>[8x]MVQASGHRRSTRGSKMVSWSVIAKIQEILQRKMVREFLAEFMSTYVMMVFGLGSVAHMVLNKKYGSYLGVNLGFGFGVTMGVHVAGRISGAHMNAAVTFANCALGRVPWRKFPVYVLGQFLGSFLAAATIYSLFYTAILHFSGGQLMVTGPVATAGIFATYLPDHMTLWRGFLNEAWLTGMLQLCLFAITDQENNPALPGTEALVIGILVVIIGVSLGMNTGYAINPSRDLPPRIFTFIAGWGKQVFSNGENWWWVPVVAPLLGAYLGGIIYLVFIGSTIPREPLKLEDSVAYEDHGITVLPKMGSHEPTISPLTPVSVSPANRSSVHPAPPLHESMALEHF

pmcAquaporins (AQPs) are integral membrane proteins facilitating the flux of water (orthodox AQPs) and/or small neutral solutes such as glycerol, arsenite, and urea (aquaglyceroporins) across the lipid bilayer of cells. The human genome encodes four aquaglyceroporins AQP3, AQP7, AQP9, and AQP10 and recently AQP7 was identified as a novel regulator of breast cancer. The model shows the typical AQP fold with six transmembrane segments and two half helices located on loop B and loop E. Furthermore, the conserved aromatic/arginine selectivity filter (ar/R) and NPA-motifs (NAA and NPS in AQP7), characteristics of the AQP family, are clear in the model.

Here, we report the single-particle cryo-EM structure of human AQP7 at 3.2 Å overall resolution in complex with the specific AQP7 inhibitor Z433927330 (4). As seen for AQP7g, the AQP7 with inhibitor (hereafter called AQP7i) adopts an octameric configuration with individual glycerol channels forming two adhering tetramers, which interact via their extracellular C loops. An unambiguous inhibitor density is observed in the glycerol channel, showing an extended shape with the kinked end exposed to the intracellular side. The inhibitor fits into the glycerol channel of AQP7 by binding near the ar/R filter (composed of Phe74, Tyr223, and Arg229) and extends to the endofacial side of the pore. The ethyl-benzoate group is accommodated in the wider pore area in the vicinity of the NPA motifs (Asn94 and Asn226). Further toward the intracellular side of the pore, the ligand forms two hydrogen bonds via its urea NH groups to the carbonyl oxygens of His92 and Ala91, situated on loop B. Closest to the cytoplasmic side of the pore, the phenyl pyrazole group is accommodated, and the nitrogen of the pyrazole ring hydrogen bonds to the side chain of Gln183, which likely positively affects the specificity and affinity of the compound. In particular, two residues located at the intracellular vestibule of AQP7i, Arg106, and Phe187, display significant shifts in comparison with the AQP7g structure, resulting in a wider channel at the intracellular side to accommodate the inhibitor. The Phe187 side chain rotates approximately 90° to avoid steric clashes with the inhibitor and instead it forms a CH–π interaction between its phenyl ring and the carbon atom of the pyrazole ring of the inhibitor. Permeation analysis revealed no water permeation when the inhibitor was bound to AQP7.> ASMQCKVILLDGSEYTC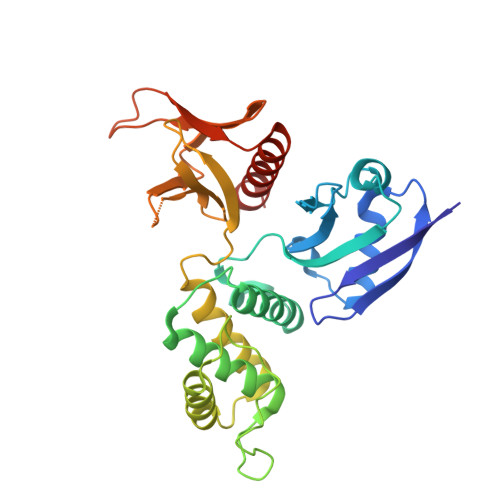DVEKRSRGQVLFDKVCEHLNLLEKDYFGLTYRDAENQKNWLDPAKEIKKQVRSGAWHFSFNVKFYPPDPAQLSEDITRYYLCLQLRDDIVSGRLPCSFVTLALLGSYTVQSELGDYDPDECGSDYISEFRFAPNHTKELEDKVIELHKSHRGMTPAEAEMHFLENAKKLSMYGVDLHHAKDSEGVEIMLGVCASGLLIYRDRLRINRFAWPKVLKISYKRNNFYIKIRPGEFEQFESTIGFKLPNHRAAKRLWKVCVEHHTFFRLL> MITFTFMSLVTSVKDYVEITHKLIEIEPLKNYTEFGAVFTYFIFSIGEFFKNFFSFSFLNNIWSIPIIIPDIASAMISEVSVLDGYFHNAFTFLETSVNTTTNPSLVIFEKFVIGIINSLFLILPTSTSHLITLRRFVMQGLEAGYMAGLGTLAGNFLWLASIILGWRFFVIPWLSLDIFRYLLGFVLLVKYIWDSSKERRMALEDLSKWKIFLLNFLLALTEQSCIYPFISNLSFGPDASILEGFPVDNYPQFLLIHGAYLLGILFGSFSLLQFTCWFWENPAFSIYLWITTKSSLKISTSSYYKILNFTFLYATMLCAIASIPYYGLDYTITNPIGLVPQDRILNQKKSQSDPDKLITETAFLNLNPTDKNSRIRDGVHARRERWKQRLIKYQAFDASTYDQGVYDFLTIEDLNYGFDRFWLRRKMRNHQIRFRLFPGPWMRSLKKQLNNPANPSLETSTKAASGPRVEFFRILFEQFYHPNFHDRAAMQTNPAEARNKFISTSPLASTESKKALNSTFSLGNINNSSTGIEGLVLTNTQATLLPTDLQTKRTIKPGLIYTNSALRKFVRNVNTRLNLKLLNSKETNLTTKYKSQFIYSKRWKSIFSKIQPLQNGTTRKSYQLFRNVAKQILVTPDAKSLKLITINQKLSLKERKLLELRTQYNNNSTLTTTAPLTLVRPLNVYLQKEEAFKRKLRYYGTMPMRKLTVGNQAPYFKALMKRGFYYYKPTLRWRKTLYVASLRRGFRKKSRKQRILVMPSNQQNFNNTLDNTKTNINQNNLANPLGGNEVPMYGADGENSLITKPTHSYTVLGKRASRYRHQIYKDVLQ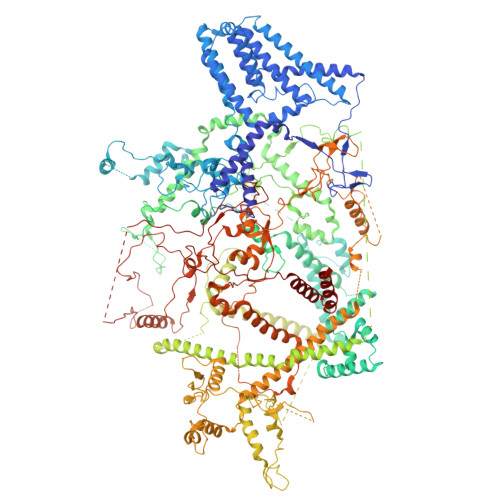HWYYTPFNRLLMKFDVDAFINRQPKSHFLTKNEERALHIRRFLLSEHYDTLRWYTYMQHYKTMKTNIGGTKSFANRAYNQQFQGTFKKIRHLFAITPKQGDFYTLKFDQPLYNDNKLKDNLYFHEELLTDYYNGTNLQTNQTSNISVNSTTTFIDNSLRTTQLPVPSSSFDIVNQSSTLIGLTTMQNALRKNVVESTLTSLNSDGEAATSQPKLNFVYSELFVKLIKECKKRIHDQTFLKNYITHRIEKREQLNQEQTKELNKRLEKLKVWLNSDKGSISKLQNTPVQDPNISSPDKVLTTAMQKAVNESISLSGIMPSDKIKTTYGNLTNAYTIKTENAILTKLNVINQLTNNETTTQKNTLIKSIGVNKIQTVLQTIITNFKSSLYNQTQLLRVKTDKDLQWWRTKQRVITKRKSARKRDRFKKQIAVVNKKLAALSKKVETEKSNLYQTLYGNYEISDYLLRNVPTGSSAVIDSTVLRKKQDNQAYLPKETNNVQFNSFVDSNNNVWQTFFAKKLRKKISSKGRRYRSLSLARYLTATRKPRLVGLDNLTKIDNITTLQGAFITKEEKQDSLNLTIQRKQELTNSLKKSQIKKRSRHSWKKRSRHQFSRNHYKYRKRHTHGNGKLRVMNKKLKKFKATNELRQWWWNSFLPRYLSNLQVNNSTLTNKNVSFKPLSNTNSVPSTNMASPTTSRNLLDNLNSSNQISTSASMNQNIVTESVKVETNQVYLPEGEKSFDITSMTTTLPFYAGWDESLKKFVVTNRLLSRRDAGLSVNNNPQEINFTNPPIQGLNEGSFLYWQTEMPFNSYNIDQFITTNQSFYAPLGWRRFEFRHSILKTWVNNTKAGNNNIKKKTLIISLKNLQPLKSSQQKQNQIKTKKLVARRIKKRYKLLKQMPNQLMYSPTGPLLTEVLPSHYISVFDQQYRLPRNRYLKRNPLKTLKKTTLLALMDSSKQTNGVNKEFTLRKRVKPRRKYHRKRFIKKDGLIFPRRTKFNTNTTLTGNALITNNVNSIEEDDLRWRPSSRTKQKRKDNTRSSAASKTKSNKRVKTNPLRLRQLRRREFQQVLKPLQRYIPQNGGFTWPGDYLRLEIVEMPKLKSINIKKTSLKQKINVQPVGIMPRKYLIEKHNIKVLKKKLSQAYSTQQLTKVVQEYKNLIQNSPPAI> MTDQNLPVTVAGLGPMGSALAAALLDRGHDVTVWNRSPGKAAPLVA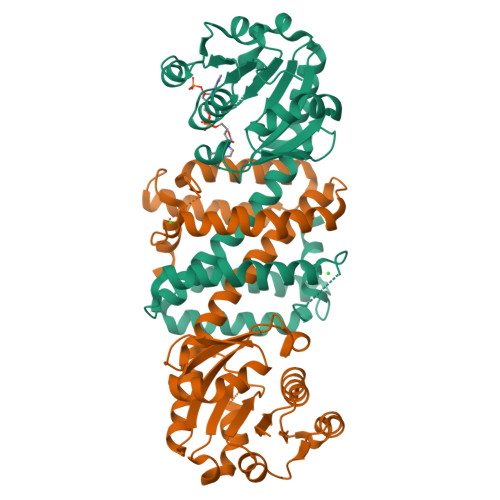KGARQADDIVDAVSASRLLVVCLADYDALYSALGPAREALRGRVVVNLNSGTPKEANEALRWAERHGTGYLDGAIMVPPAMVGHPGSVFLYSGSAEVFEEYKETLAGLGDPVHLGTEAGLAVLYNTALLSMMYSSMNGFLHAAALVGSAGVPAAEFTKLAVDWFLPAVIGQIIKAEAPTIDEGVYPGDAGSLEMNVTTLKHIIGTSQEQGVDTEIPVRNKELLDRAVAAGFGESSYYSVIELWR;> MTDQNLPVTVAGLGPMGSALAAALLDRGHDVTVWNRSPGKAAPLVAKGARQADDIVDAVSASRLLVVCLADYDALYSALGPAREALRGRVVVNLNSGTPKEANEALRWAERHGTGYLDGAIMVPPAMVGHPGSVFLYSGSAEVFEEYKETLAGLGDPVHLGTEAGLAVLYNTALLSMMYSSMNGFLHAAALVGSAGVPAAEFTKLAVDWFLPAVIGQIIKAQAPTIDEGVYPGDAGSLEMNVTTLKHIIGTSQEQGVDTEIPVRNKELLDRAVAAGFGESSYYSVIELWR[[(2S,3aS,5S,6R,6aS)-2-dodecyl-6-oxidanyl-3a,5,6,6a-tetrahydrofuro[2,3-d][1,3]dioxol-5-yl]methoxy-oxidanyl-phosphoryl] [(2R,3S,4R,5R)-5-(6-aminopurin-9-yl)-3,4-bis(oxidanyl)oxolan-2-yl]methyl 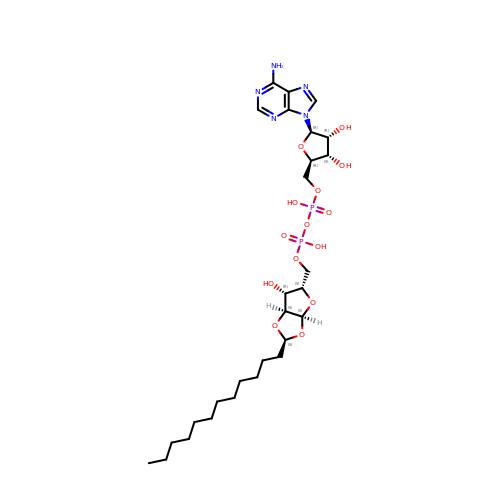hydrogen phosphate | C28 H47 N5 O14 P2 | KJBRVZZXXRAVKC-XBVYZWAMSA-N> MVVLKCPVCNGDVNVPDDALPGEIVEHECGAQLEVYNDHGRLALR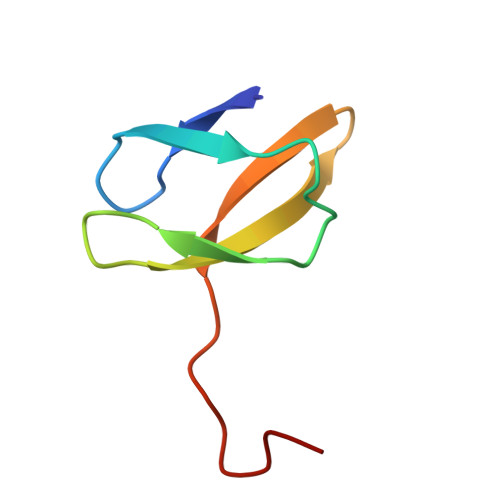LAEQVGEDWGE> MSKYSQDVLQLLYKNKPNYISGQSIAESLNISRTAVKKVIDQLKLEGCKIDSVNHKGHLLQQLPDIWYQ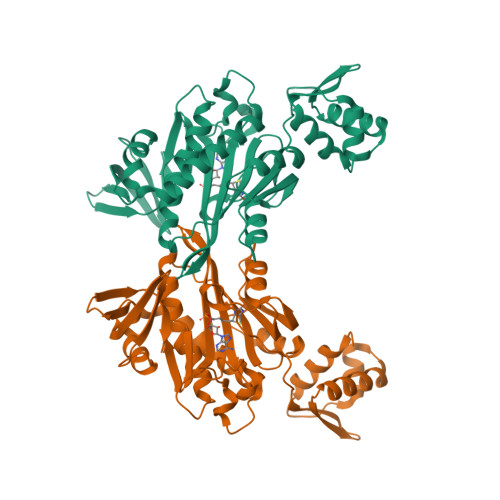GIIDQYTKSSALFDFSEVYDSIDSTQLAAKKSLVGNQSSFFILSDEQTKGRGRFNRHWSSSKGQGLWMSVVLRPNVAFSMISKFNLFIALGIRDAIQHFSQDEVKVKWPNDIYIDNGKVCGFLTEMVANNDGIEAIICGIGINLTQQLENFDESIRHRATSIQLHDKNKLDRYQFLERLLQEIEKRYNQFLTLPFSEIREEYNAASNIWNRTLLFTENDKQFKGQAIDLDYDGYLIVRDEAGESHRLISADIDF>MRVLALSAVFLVASIIGMPAVAKEWQENKSWNAHFTEHKSQGVVVLWNENKQQGFTNNLKRANQAFLPASTFAIPNSLIALDLGVVKDEHQVFKWDGQTRDIATWNRDHNLITAMKYSVVPVYQEFARQIGEARMSKMLHAFDYGNEDISGNVDSFWLDGGIRISATEQISFLRKLYHNKLHVSERSQRIVKQAMLTEANGDYIIRAKTGYSTRIEPKIGWWVGWVELDDNVWFFAMNMDMPTSDGLGLRQAITKEVLKQEKIIP[2x]

Of the serine carbapenemases, the OXA family of carbapenem-hydrolyzing class D β-lactamases (CHDLs) represent a formidable treatment challenge. OXA-48 is referred to as the “phantom menace” or “hidden threat” as clinical isolates producing OXA-48 are often difficult to detect, missed by routine diagnostics, and the blaOXA-48 gene is localized to a plasmid that disseminates rapidly. The major active site residues in OXA-48 that contribute to β-lactam hydrolysis are the catalytic serine residue, S70 that forms a covalent/acyl bond with the substrates, and K73, which needs to be carbamylated in OXA-β-lactamases to aid in the deacylation reaction involving a water molecule. When comparing different carbapenems, OXA-48 most efficiently hydrolyzes imipenem with a kcat/Km value of 370 mM−1s−1, whereas hydrolysis of meropenem and ertapenem are appreciably less at 6 mM−1s−1 and 1 mM−1s−1, respectively and doripenem turnover is not detectable.

To probe the molecular basis for carbapenem selectivity, we determined the crystal structure of the K73A deacylation-deficient mutant of OXA-48 in complex with doripenem at 1.5 Å resolution. We obtained a 1.5 Å resolution data set of the OXA-48 K73A variant co-crystallized with doripenem with two OXA-48 molecules (molecule A and B) in the asymmetric unit. In molecule A, doripenem’s sulfur atom adjacent to the R2 pyrrolidine ring is in the R-configuration (Δ1R). In molecule B, the cavity resulting from this mutation was occupied, in part, by a full occupied chloride ion; in molecule A, the W157 adopts a different conformation that is made possible by the K73A cavity-introducing mutation. There is a covalent (acyl) bond between doripenem and S70. The β-lactam carbonyl oxygen occupies the nearby oxyanion hole comprised of backbone nitrogen atoms of S70 and Y211. One of the oxygens of the carboxylate moiety of doripenem is interacting with the side chain of R250 thus forming a salt bridge. The methyl moiety attached to the C1 position of the core pyrroline ring is making van der Waals interactions with the CD2 atoms of Y211 (3.8 Å distance for both doripenem molecules). The hydroxyethyl moiety is in the same orientation in both doripenem molecules; this moiety is not making direct hydrogen bonds with the protein but is making van der Waals interactions with residues Y105, V120, and L158. Despite all these caveats and uncertainties, our structural results point to an importantrole for OXA-48 residues Y211 and V120 for the poor activity of C1-methyl containing carbapenems and doripenem in particular.>XGEIKAIAQEIKAIAKEIKAIAWEIKAIAQGX[6x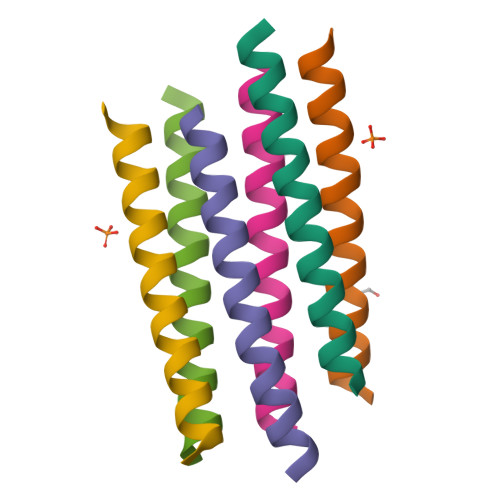]> DCSSGWSSYEGHCYKVFKQSKTWADAESFCTKQVNGGHLVSIESSGEADFVGQLIAQKIKSAKIHVWIGLRAQNKEKQCSIEWSDGSS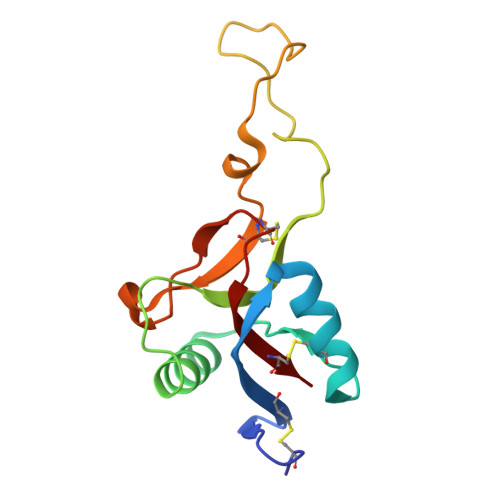ISYENWIEEESKKCLGVHIETGFHKWENFYCEQQDPFVCEA> ALPQTVRIGTDTTYAPFSSKDAKGEFIGFDIDLGNEMCKRMQVKCTWVASDFDALIPSLKAKKIDAIIASLSITDKRQQEIAFSDKLYAADSRLIAAKGSPIQPTLESLKGKHVGVLQGSTQEAYANDNWRTKGVDVVAYANQDLIYSDLTAGRLDAALQDEVAASEGFLKQPAGKEYAFAGPSVKDKKYFGDGTGVGLR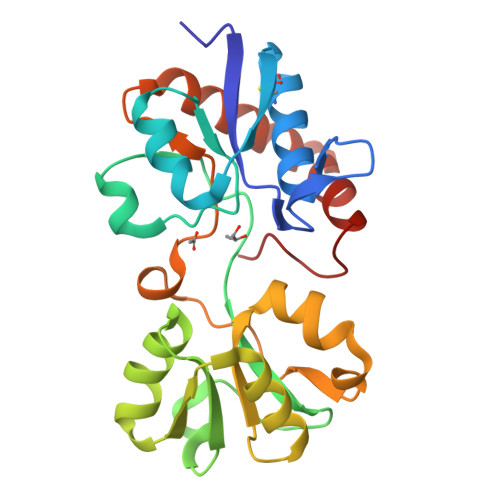KDDTELKAAFDKALTELRQDGTYDKMAKKYFDFNVYGD>LAMVDNLQGDSGRGYYLEMLIGTPPQKLQILVDTGSSNFAVAGTPHSYIDTYFDTERSSTYRSKGFDVTVKYTQGSWTGFVGEDLVTIPKGFN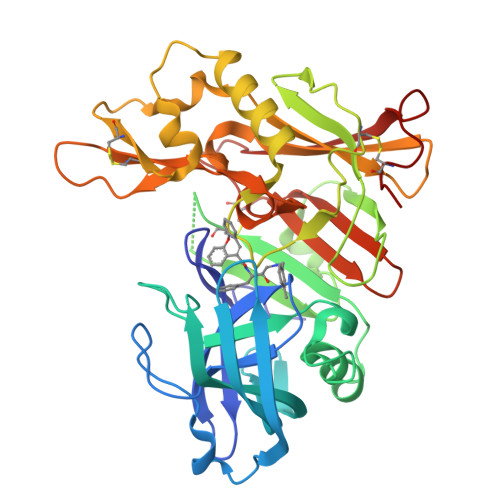TSFLVNIATIFESENFFLPGIKWNGILGLAYATLAKPSSSLETFFDSLVTQANIPNVFSMQMCGAGLPVAGSGTNGGSLVLGGIEPSLYKGDIWYTPIKEEWYYQIEILKLEIGGQSLNLDCREYNADKAIVDSGTTLLRLPQKVFDAVVEAVARASLIPEFSDGFWTGSQLACWTNSETPWSYFPKISIYLRDENSSRSFRITILPQLYIQPMMGAGLNYECYRFGISPSTNALVIGATVMEGFYVIFDRAQKRVGFAASPCAEIAGAAVSEISGPFSTEDVASNCVPA[4x]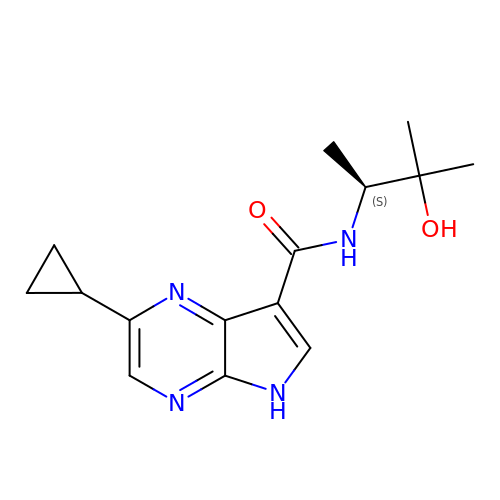2-cyclopropyl-N-[(2S)-3-hydroxy-3-methylbutan-2-yl]-5H-pyrrolo[2,3-b]pyrazine-7-carboxamide | C15 H20 N4 O2 | ODYYFDDUIDLRBK-QMMMGPOBSA-N(2R,4S)-N-BUTYL-4-HYDROXY-2-METHYL- 4-((E)-(4AS,12R,15S,17AS)-15-METHYL -14,17-DIOXO-2,3,4,4A,6,9,11,12,13, 14,15,16,17,17A-TETRADECAHYDRO-1H-5 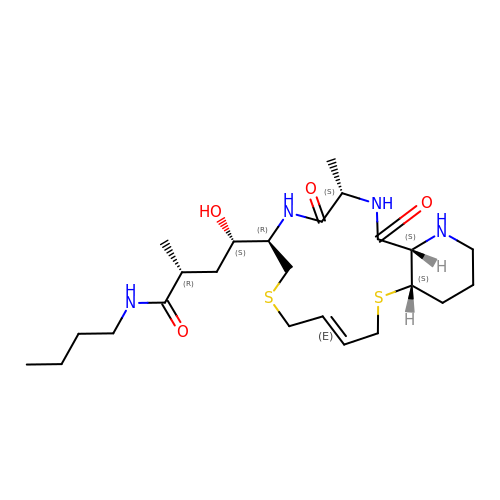,10-DITHIA-1,13,16-TRIAZA-BENZOCYCL OPENTADECEN-12-YL)-BUTYRAMIDE | C24 H42 N4 O4 S2 | FIWCVIADXWJIGF-NFXSCPKSSA-N>[2x]GSHDSGDKITATSSLKTPIVNRAITESEVLAAQKAWGEALVAISTTYDAKGKASAKALAEKVIDDAYGYQFGPVLFKPTLAISPRTFRTTRAGALAYFVGDDKAFPEDKGFALSSWRKVEIKNAAIFITGNTATTMGNVIITDKQGKATTVDKTWQFLKDDHGKLRIITHHSSLPYEQ

In the present study, we report a novel type of CAs that has been characterized in the eukaryotic microalga Bigelowiella natans and the cyanobacterium Anabaena sp. PCC7120. Taken together, these results suggested that the COG4337 proteins are metal-free enzymes that catalyze the hydration of CO2 to HCO3-, but not the reverse reaction. Each domain formed a cone-shaped barrel structure comprising three α-helices and a four-stranded antiparallel β-sheet, which were almost identical across the COG4337 domains of Bn86287 and all2909. We thus concluded that COG4337 proteins should be treated as a new variant of ι-class CAs.

To further analyze the metal-free catalytic mechanism of COG4337 proteins, crystal structures of Bn86287 and all2909 were determined. The substrate (bicarbonate) and inhibitor (iodide ion) were found in a bent finger-like cavity of the cone-shaped barrel. As expected from the biochemical assays described above, electron densities corresponding to metals were not detected in the cavity. Notably, Lys180 in all2909 was found at the analogous position of Tyr224/388/552 in Bn86287. To evaluate the functional importance of the cavity-forming residues, we performed point mutation analysis, wherein Thr106, Tyr124, Lys180, His197, and Ser199 were substituted by alanine in all2909, and Thr486, Tyr503, Tyr552, His584, and Ser586 were replaced by alanine using a recombinant protein of the third COG4337 domain (431–607 amino acids) in Bn86287. In all2909, the substitution of Lys180 did not affect the CA activity, while the other four mutations resulted in complete inactivation. Considering that hydroxyl groups of Thr106/159/322/486 (residue numbers in all2909/1st/2nd/3rd domain of Bn86287) and Tyr124/176/339/503 were found at a distance of 2.5 to 3.5 Å from an oxygen of HCO3- and at a distance of 3.2 to 3.7 Å from an iodide ion, these hydroxyl groups would most likely mediate the deprotonation of active site water. The deprotonation process could also be assisted by the main chain nitrogen of Thr106/159/322/486 and the hydroxyl group of Ser199/258/422/586 that is positioned within hydrogen bond distance to Thr106/159/322/486. The results of size exclusion chromatography with multi-angle static light scattering (SEC-MALS) system showed that Bn86287 exists as dimers but all2909 exists as tetramers in solution. Analysis with the PISA (Protein Interfaces, Surfaces and Assemblies) software estimated that a tetramer of all2909 was assembled by a head-to-head interaction of two dimeric units.> MVIGLSTGSDDDDVEVIGGVDPRLIAVQENDSDESSLTDLVEQPAKVMRIGTMIKQLLEEVRAAPLDEASRNRLRDIHATSIRELEDGLAPELREELDRLTLPFNEDAVPSDAELRIAQAQLVGWLEGLFH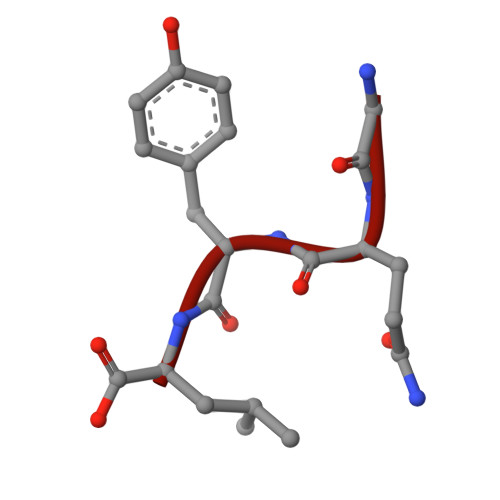GIQTALFAQQMAARAQLQQMRQGALPPGVGKSGQHGHGTGQYL>DSISLSLINEGPSYASKVSVGSNKQQQTVIIDTGSSDFWVVDSNAQCGKGVDCKSSGTFTPSSSSSYKNLGAAFTIRYGDGSTSQGTWGKDTVTINGVSITGQQIADVTQTSVDQGILGIGYTSNEAVYDTSGRQTTPNYDNVPVTLKKQGKIRTNAYSLYLNSPSAETGTIIFGGVDNAKYSGKLVAEQVTSSQALTISLASVNLKGSSFSFGDGALLDSGTTLTYFPSDFAAQLADKAGARLVQVARDQYLYFIDCNTDTSGTTVFNFGNGAKITVPNTEYVYQNGDGTCLWGIQPSDDTILGDNFLRHAYLLYNLD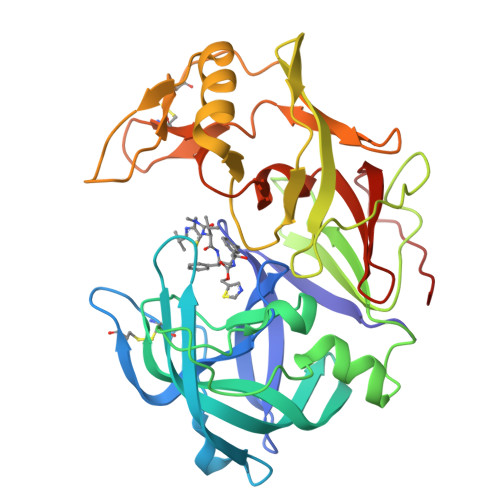ANTISIAQVKYTTDSSISAV[2x]> MEVTHKQFDLSGFLPDQAPDTLKSGAISRGFNVKPTILGWEKSGGFRETNTAPTNEKDFIFFWSPAIGDNRWFSGGDKTVQQVEGNVVSDVSRTGGYTAAAAARWNAVNFNGVLLMNNELDSPQYLAASGKLEDFPNLPSNVRFRTVAVYKNFILGLGVNFGSG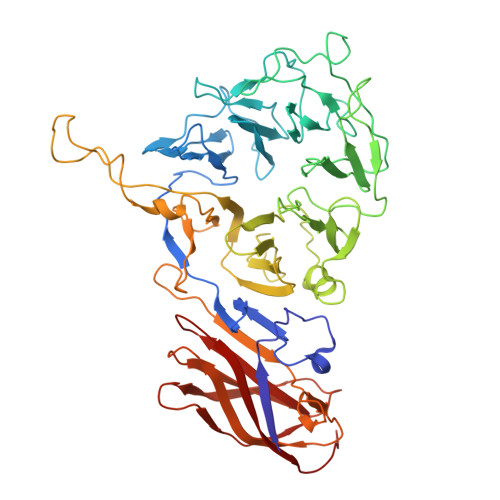FLDDEIYWSHQADPGTMPPNWDYANAASDSGRTPLPSEGYCVTSEELGSMNIVYKSDSIWTMQLIGGQWIFRFENKFPGQGILNKKSVVSFEGKHFVVTQKDIIVHDGYQVRSVADKRVRNFFFTDMNSDYFERVFVVKDPRVAEVYVFYPSKNSVDGLCDRALVWNWRDDVWSLLNLRPLKHAAYGYEITGVSITWDNFVGGWESTGLWQADEDVAKYAPVLHYSFRDVPKLLAPTPQALFIDEEIEAVWEREDIVIGSISRDGVPYQDYERNKSVSSISFDVDTTEPFDVYIGYKGSLEDSVEWEFAGTVNPMEDKRLFCLLTAGLFSMRIISKAQTFILRSYKITYEFAGEMWA Here we elucidate the structural and molecular determinant(s) of target specificity of histidine vs. lysine in the active site of SETD3. On the substrate-binding surface, the residues are diverse, reflecting the fact that the three enzymes act on three very distinct substrates—the large subunit of Rubisco by LSMT, RelA subunit of nuclear factor NFκB by SETD6, and actin by SETD3—with limited sequence similarity immediately surrounding the methylation target. To facilitate the methyl transfer reaction, SETD3 provides a local environment that promotes deprotonation of the target nitrogen N3 of histidine (and concomitant protonation of N1). Most (if not all) SAM-dependent MTases use the classic SN2 reaction mechanism, which requires the target nitrogen be in a deprotonated state.

Third, to verify that the target histidine, before and after the methyl transfer reaction, can adopt two different conformations in the active site, we reduced the concentration of SAM in the reaction, which resulted in a mixture of methylated and unmethylated peptides, and followed with crystallization. Indeed, the active-site density for the histidine residue can be modeled by two ring conformations with a rotation of ~105°, whereas the conformations of residues lining the active-site pocket remain unchanged. The position of the target N3 atom and its relative distance to the cofactor in the two conformations are virtually identical. We think the primary reason for the rotation is to switch the proton from N3-H to N1-H, ensuring the target atom N3 is deprotonated prior to the methyl transfer. As a result, the deprotonated N3 nitrogen carrying a lone pair of electrons attacks, in a nucleophilic manner, the positively charged methylsulfonium of SAM.

>GPLGSMGKKSRVKTQKSGTGATATVSPKEILNLTSELLQKCSSPAPGPGKEWEEYVQIRTLVEKIRKKQKGLSVTFDGKREDYFPDLMKWASENGASVEGFEMVNFKEEGFGLRATRDIKAEELFLWVPRKLLMTVESAKNSVLGPLYSQDRILQAMGNIALAFHLLCERASPNSFWQPYIQTLPSEYDTPLYFEEDEVRYLQSTQAIHDVFSQYKNTARQYAYFYKVIQTHPHANKLPLKDSFTYEDYRWAVSSVMTRQNQIPTEDGSRVTLALIPLWDMCNHTNGLITTGYNLEDDRCECVALQDFRAGEQIYIFYGTRSNAEFVIHSGFFFDNNSHDRVKIKLGVSKSDRLYAMKAEVLARAGIPTSSVFALHFTEPPISAQLLAFLRVFCMTEEELKEHLLGDSAIDRIFTLGNSEFPVSWDNEVKLWTFLEDRASLLLKTYKTTIEEDKSVLKNHDLSVRAKMAIKLRLGEKEILEKAVKSAAVNREYYRQQMEEKAPLPKYEESNLGLLESSVGDSRLPLVLRNLEEEAGVQDALNIREAISKAKATENGLVNGENSIPNGTRSENESLNQESKRAVEDAKGSSSDSTAGVKE[2x];>TLKYPIEHGIVTNWD[2x]>MSKTAKRVALVGDASFYVGPSLARELARREHNLVLGDPAEGLVDELTALGVEVEAVLGVRNLADPESAQKLVAAAQERFGRIDSAAAFSGRVVTGKFLDSTLEDLHSVVQGCLEAPYHFLKAVVPVMVEQGDGQVLVMT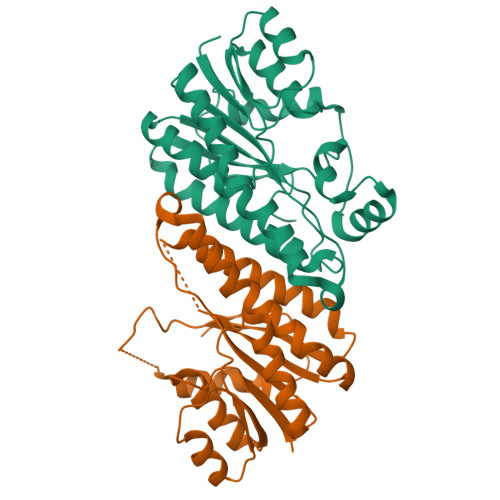SATAARPSRGASLYSSARAGATMMVKNVAAEVARNGVQVNAVGTNFMDFPEFLRASGANDPEIRARIEAAVPLGRLGTVEEFASFCMPFIDGTSKFTTGQFIAYAGGWA[4x]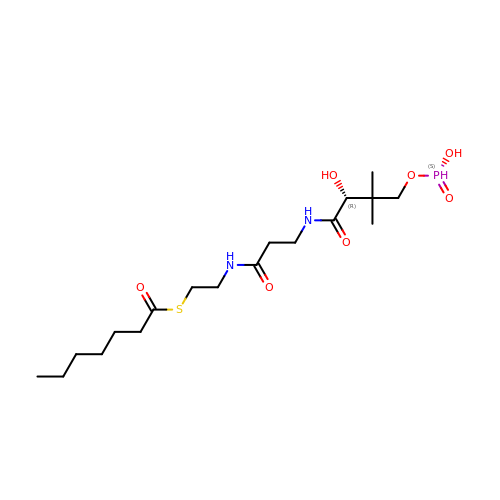S-(2-{[N-(2-HYDROXY-4-{[HYDROXY(OXIDO)PHOSPHINO]OXY}-3,3-DIMETHYLBUTANOYL)-BETA-ALANYL]AMINO}ETHYL) HEPTANETHIOATE | C18 H35 N2 O7 P S | IPSBILXXAVXCDA-INIZCTEOSA-N~{N}-[3-[1-[[4-[5-[(4-hydroxyphenyl)methyl]-6-oxidanylidene-2-phenyl-1~{H}-pyrazin-3-yl]phenyl]methyl]piperidin-4-yl]-2-oxidanylidene-1~{H}-benzimidazol-5-yl]propanamide 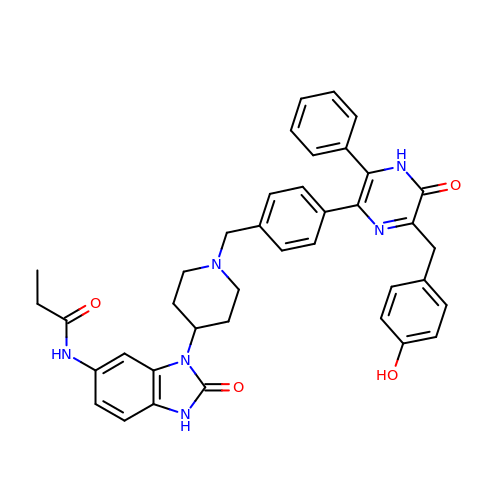| C39 H38 N6 O4 | LMPCSGMPKCSYTR-UHFFFAOYSA-N>AGADEERAETARLSSFIGAIAIGDLVKSTLGPKGMDKILLSSGRDASLMVTNDGATILKNIGVDNPAAKVLVDMSRVQDDEVGDGTTSVTVLAAELLREAESLIAKKIHPQTIIAGWREATKAARQALLNSAVDHGSDEVKFRQDLMNIAGTTLSSKLLTHHKDHFTKLAVEAVLRLKGSGNLEAIHVIKKLGGSLADSYLDEGFLLDKKIGVNQPKRIENAKILIANTGMDTDKIKIFGSRVRVDSTAKVAEIEHAEKEKMKEKVERILKHGINCFINRQLIYNYPEQLFGAAGVMAIEHADFVGVERLALVTGGEIASTFDHPELVKLGSCKLIEEVMIGEDKLIHFSGVALGEACTIVLRGATQQILDEAERSLHDALCVLAQTVKDSRTVYGGGCSEMLMAHAVTQLASRTPGKEAVAMESYAKALRMLPTIIADNAGYDSADLVAQLRAAH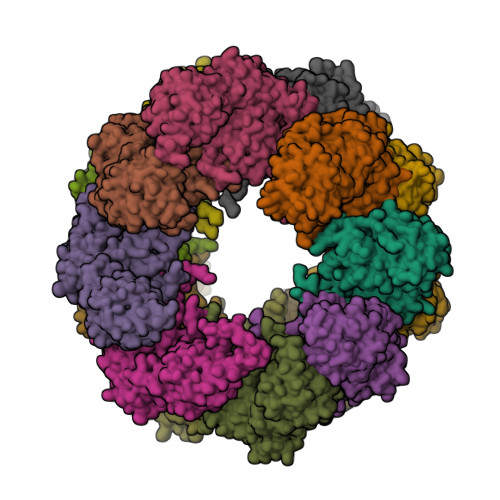SEGKTTAGLDMKEGTIGDMSVLGITESFQVKRQVLLSAAEAAEVILRVDNIIKAAPR[16x]>[14x]MQQGQMAYDRAITVFSPDGRLFQYEYAREAVKKGSTALGMKFANGVLLISDKKVRSRLIEQNSIEKIQLIDDYVAAVTSGLVADARVLVDFARISAQQEKVTYGSLVNIENLVKRVADQMQQYTQYGGVRPYGVSLIFAGIDQIGPRLFDCDPAG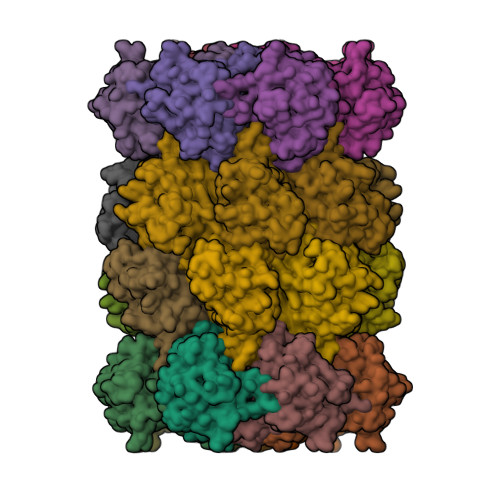TINEYKATAIGSGKDAVVSFLEREYKENLPEKEAVTLGIKALKSSLEEGEELKAPEIASITVGNKYRIYDQEEVKKFL;>[14x]MNQTLETGTTTVGITLKDAVIMATERRVTMENFIMHKNGKKLFQIDTYTGMTIAGLVGDAQVLVRYMKAELELYRLQRRVNMPIEAVATLLSNMLNQVKYMPYMVQLLVGGIDTAPHVFSIDAAGGSVEDIYASTGSGSPFVYGVLESQYSEKMTVDEGVDLVIRAISAAKQRDSASGGMIDVAVITRKDGYVQLPTDQIESRIRKLGLIL>MASQPNSSAKKKEEKGKNIQVVVRCRPFNLAERKASAHSIVECDPVRKEVSVRTGGLADKSSRKTYTFDMVFGASTKQIDVYRSVVCPILDEVIMGYNCTIFAYGQTGTGKTFTMEGERSPNEEYTWEEDPLAGIIPRTLHQIFEKLTDNGTEFSVKVSLLEIYNEELFDLLNPSSDVSERLQMFDDPRNKRGVIIKGLEEITVHNKDEVYQILEKGAAKRTTAATLMNAYSSCSHSVFSVTIHMKETTIDGEELVKIGKLNLVDLAGSENIGRSG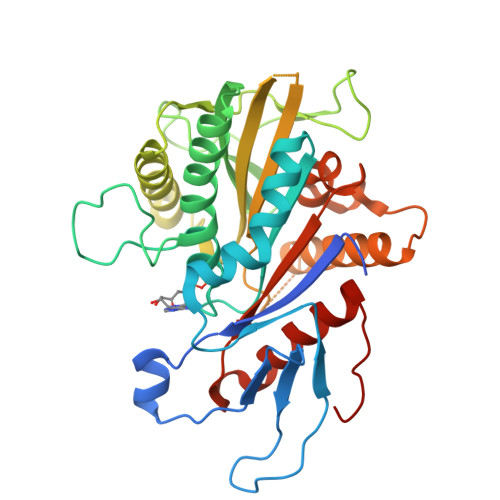AVDKRAREAGNINQSLLTLGRVITALVERTPHVPYRESKLTRILQDSLGGRTRTSIIATISPASLNLEETLSTLEYAHRAKNILNKPEVNQK[3x]5-{[AMINO(IMINO)METHYL]AMINO}-2-(SULFANYLMETHYL)PENTANOIC ACID | C7 H15 N3 O2 S 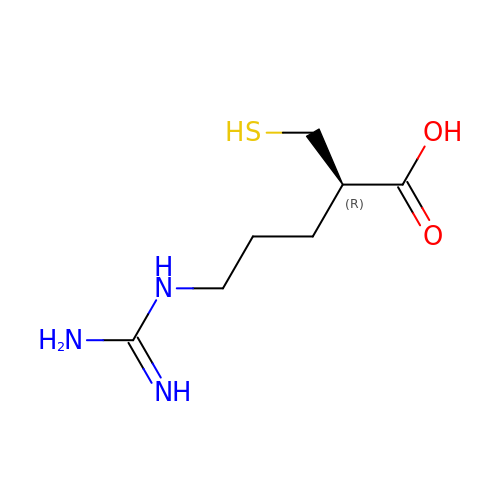| JOVIPJZDTSYNNW-YFKPBYRVSA-N>MINYGVVGVGYFGAELARFMNMHDNAKITCVYDPENGENIARELQCINMSSLDALVSSKLVDCVIVATPNYLHKEPVIKAAKNKKHVFCEKPIALSYEDCVDMVKACKEAGVTFMAGHIMNFFNGVQYARKLIKEGVIGEILSCHTKRNGWENKQERLSWKKMKEQSGGHLYHHIHELDCVQHLLGEIPETVTMIGGNLAHSGPGFGNEDDMLFMTLEFPSGKLATLEWGSAFNWPEHYVIINGTKGSIKIDMQETAGSLR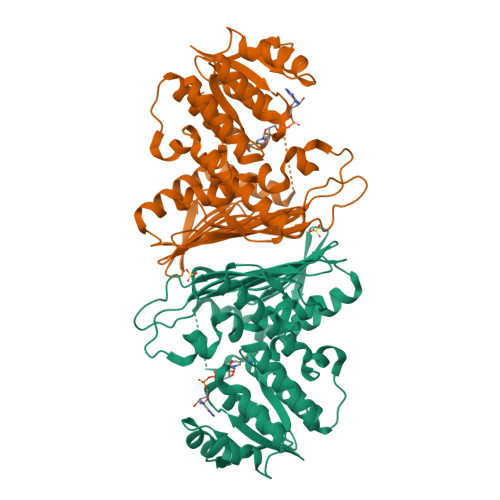IGGQTKHFLVHETQEEDDDRRKGNMTSEMDGAIAYGHPGKKTPLWLASLIRKETLFLHNILCGAKPEEDYIDLLNGEAAMSAIATADAATLSRSQDRKVKISEIIKHTSVM[2x]> CSCSSLMDKECVYFCHLDIIW;> EERGFPPDRATPLLQTAEIMTPPTKTLWPKGDYKDDDDKLAPAEVPKGDRTAGSPPRTISPPPCQGPIEIKETFKYINTVVSCLVFVLGIIGNSTLLRIIYKNKCMRNGPNILIASLALGDLLHIVIDIPINVYKLLAEDWPFGAEMCKLVPFIQKASVGITVLSLCALSIDRYRAVASWSRIKGIGVPKWTAVEIVLIWVVSVVLAVPEAIGFDIITMDYKGSYLRICLLHPVQKTAFMQFYKTAKDWWLFSFYFCLPLAITAFFYTLMTCEMLRKKSGMQIALNDHLKQRREVAKTVFCLVLVFALCWLPLHLSRILKLTLYNQNDPNRCELLSFLLVLDYIGINMASLNSCINPIALYLVSKRFKNCFKSCLCCWCQSFEEKQSLEEKQSCLKFKANDHGYDNFRSSNKYSSSGSGGGGSGGSSSGGVFTLEDFVGDWEQTAAYNLDQVLEQGGVSSLLQNLAVSVTPIQRIVRSGENALKIDIHVIIPYEGLSADQMAQIEEVFKVVYPVDDHHFKVILPYGTLVIDGVTPNMLNYFGRPYEGIAVFDGKKITVTGTLWNGNKIIDERLITPDGSMLFRVTINSGGSGGGGSGGSSSGGLEVLFQ

The endothelin ETB receptor is a promiscuous G-protein coupled receptor that is activated by vasoactive peptide endothelins. By contrast, the ETB receptor primarily induces vasorelaxation via the nitric oxide-mediated pathway, and it acts as a clearance receptor that removes circulating ET-1 via the lysosomal pathway Bremnes et al., 2000. The ETB receptor is known to be a promiscuous GPCR, capable of activating multiple types of G-proteins Inoue et al., 2019; Doi et al., 1999. Here, we report the 2.8 Å-resolution cryo-electron microscopy (cryo-EM) structure of the human ETB-Gi signaling complex bound to ET-1, revealing the unique mechanisms of receptor activation and G-protein coupling.

We refined with a mask on the receptor and obtained the receptor structure with a nominal resolution of 3.1  Å. The agonist ET-1 is well resolved. The extracellular half of the receptor superimposes well on the ET-1-bound crystal structure, and ET-1 interacts closely with the receptor in a similar manner. The ligand binding pocket is essentially similar in both the crystal structure of the receptor alone and in the Gi protein complex. However, the W3366.48 rotamer, which comprises the bottom of the ligand-binding pocket, differs, thereby leading to the activation of the intracellular side of the receptor. The downward movement of the residues is larger in the ETB-Gi complex than in the ET-1-bound crystal structure, which consequently results in the outward displacement of the intracellular portion of the transmembrane helix (TM) 6 by 6.8 Å as compared to the apo state, and by 5.1 Å as compared to the ET-1-bound crystal structure. Upon receptor activation, the ionic lock between D1983.49 and R1993.50 is broken, and R1993.50 becomes oriented towards the intracellular cavity, similar to other GPCRs Zhuang et al., 2022; Rasmussen et al., 2011; Ring et al., 2013; Cherezov et al., 2007; Manglik et al., 2012; Huang et al., 2015. In contrast, the N7.49P7.50xxY7.53 motif is altered to N7.49P7.50xxL7.53Y7.54, where Y7.53 is replaced by L3867.53. As L3867.53 is a hydrophobic residue, it cannot form a polar interaction, and hence in the ETB-Gi complex, TM7 is not displaced inwardly. Moreover, the intracellular portion of TM7 is displaced downward by 2.8 Å.>[4x]MGSSHHHHHHGSGVKTENNDHINLKVAGQDGSVVQFKIKRHTPLSKLMKAYCERQGLSMRQIRFRFDGQPINETDTPAQLEMEDEDTIDVFQQQTGGSKFSNITIKNFRNFEKVNINLDNKNVIFGMNDIGKTNFLYALRFLLDKEIRKFGFNKSDYHKHDTSKKIEIILTLDLSNYEKDEDTKKLISVVKGARTSANADVFYIALESKYDDKELYGNIILKWGSELDNLIDIPGRGNINALDNVFKVIYINPLVDLDKLFAQNKKYIFEESQGNESDEGILNNIKSLTDQVNQQIGEMTIIKGFQQEITSEYRSLKKEEVSIELKSEMAIKGFFSDIIPYIKKDGDSNYYPTSGDGRRKMLSYSIYNYLAKKKYEDKIVIYLIEEPEISLHRSMQIALSKQLFEQSTYKYFFLSTHSPELLYEMDNTRLIRVHSTEKVVCSSHMYNVE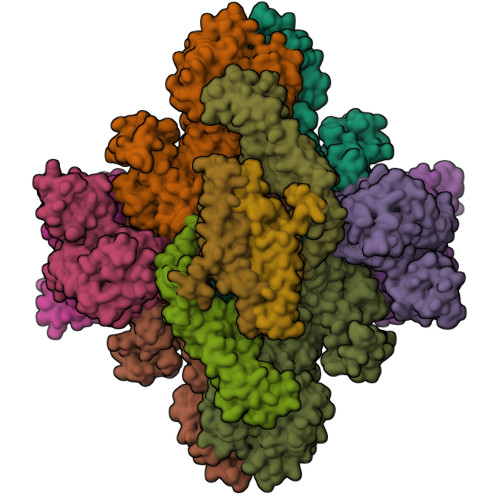EAYGSVKKKLNKALSSALFAERVLLIEGPSEKILFEKVLDEVEPEYELNGGFLLEVGGTYFNHYVCTLNDLGITHIIKTDNDLKSKKGKKGVYELLGLNRCLNLLGRENLDEITIDIPEDIKGKKKKERLNERKKEIFKQYKNEVGEFLGERIYLSEIDLENDLYSAIGESMKRIFENEDPVHYLQKSKLFNMVELVNNLSTKDCFDVFEHEKFACLKELVGSDRG;>MSREQIIKDGGNILVTAGAGSGKTTILVSKIEADLKENKTHYSIAAVTFTNKAAKEIEGRLGYSSRGNFIGTNDGFVESEIIRPFIKDAFGNDYPDNFTAEYFDNQFASYDKGLQVLKYQNILGTYSNPKKNFKFQLALDILKKSLVARQYIFSKYFKIFIDEYQDSDKDMHNLFMYLKDQLKIKLFIVGDPKQSIYIWRGAEPENFNGLIENSTDFNKYHLTSNFRCCQDIQNYSNLFNEETRSLIKEKNEVQNVISIADDMPISDILLKLTEEKQVLNIEAELVILVRRRNQAIEIMKELNEEGFNFIFIPQTPLDRATPNATLLKEVIKYVKNDRYSIYDLAAEIVGNLSSREIKEIQKIINELLVPNINQVLINQVLINLFAKLEITLDTREITAFTEVMMTNEFDIAFDTNEYLHKIFTVHSAKGLEFNQVIITASDYNVHYNRDTNEHYVATTRAKDKLIVIMDNKKYSDYIETLMKELKIKNIIKSI[4x];>[8x]MKLIGIKTSNCFLVSDNIEGKRYFHSQLDELLFDGKRATETYKSDWFKLEKEPSVIEKQMPAKKINHRYELKEGFQESELTPKVIKASYIGEDSEYYEVKGLYDLKFEEIPQQNEKIEFEMNVIEEIDGELKLQSHNFNLNYNLLDRIQTHPMLLETKPCYLSQEESYKIIRNHIKANINPKFARITSDYDFCLTVVKVLELYKPHEYIVDLNAMYKRRKPKLEKRFQTKREVEIYKVAPKAYQSYPIVEPFSGKDVEDLKSNIKKFLDDLMAKINEPLVECKCCKGRGVILNEN N-hydroxy-N~2~-(2-hydroxyethyl)-N~2~-[(4-methoxyphenyl)sulfonyl]glycinamide 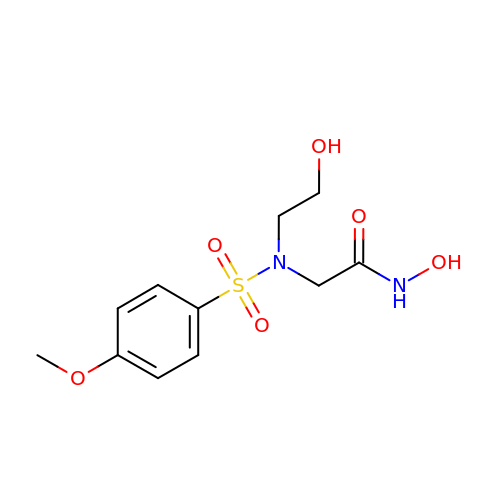| C11 H16 N2 O6 S | IVGHGMHNUBCTDC-UHFFFAOYSA-N> EPIKIMLKPGKDGPKLRQWPLTKEKIEALKEICEKMEKEGQLEEAPPTNPYNTPTFAIKKKDKNKWRMLIDFRELNKVTQDFTEIQLGIPHPAGLAKKRRITVLDVGDAYFSIPLHEDFRPYTAFTLPSVNNAEPGKRYIYKVLPQGWKGSPAIFQHTMRQVLEPFRKANKDVIIIQYMDDILIASDRTDLEHDRVVLQLKELLNGLGFSTPDEKFQKDPPYHWMGYELWPTKWKL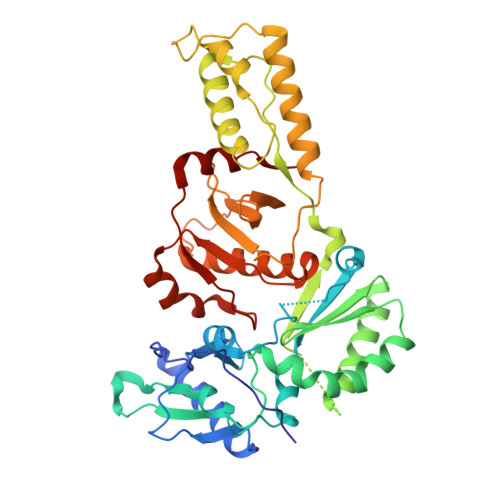QKIQLPQKEIWTVNDIQKLVGVLNWAAQLYPGIKTKHLCRLISGKMTLTEEVQWTELAEAELEENRIILSQEQEGHYYQEEKELEATVQKDQDNQWTYKIHQEEKILKVGKYAKVKNTHTNGIRLLAQVVQKIGKEALVIWGRIPKFHLPVEREIWEQWWDNYWQVTWIPDWDFVSTPPLVRLAFNLVGD>MKGRLIEVTEEELKKHNKKDDCWICIRGFVYNVSPYMEYHPGGEDELMRAAGSDGTELFDQVHRWVNYESMLKECLVGRMAIKPAVLK[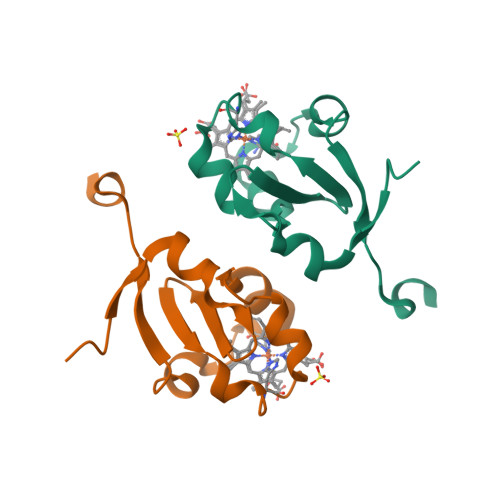2x]> MVAPLSVQGNKILANGQPASFSGMSLFWSNTEWGGEKYYNAQVVSWLKSDWNAKLVRAAMGVEDEGGYLTDPANKDRVTQVVDAAIANDMYVIIDWHSHNAHQYQSQAIAFFQEMARKYGANNHVIYEIYNEPLQVSWSNTIKPYAQAVIAAIRAIDPDNLIIVGTPTWSQDVDVAANDPITGYQNIAYTLHFYAGTHGQYLRDKAQTALNRGIALFVTEWGSVNANGDGAVANSETNAWVSFMKTNHISNANWALNDKVEGASALVPGASANGGWVNSQLTASGALAKSIISGWPSYLEH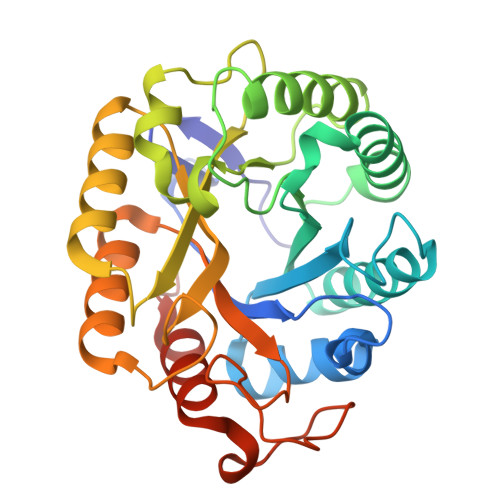HHHHH>[2x]KFPRVKNWEVGSITYDTLSAQAQQDGPCTPRRCLGSLVFPRKLQGRPSPGPPAPEQLLSQARDFINQYYSSIKRSGSQAHEQRLQEVEAEVAATGTYQLRESELVFGAKQAWRNAPRCVGRIQWGKLQVFDARDCRSAQEMFTYICNHIKYATNRGNLRSAITVFPQRCPGRGDFRIWNSQLVRYAGYRQQDGSVRGDPANVEITELCIQHGWTPGNGRFDVLPLLLQ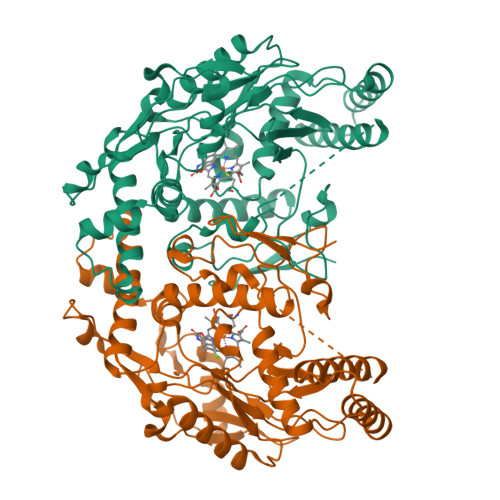APDEPPELFLLPPELVLEVPLEHPTLEWFAALGLRWYALPAVSNMLLEIGGLEFPAAPFSGWYMSTEIGTRNLCDPHRYNILEDVAVCMDLDTRTTSSLWKDKAAVEINVAVLHSYQLAKVTIVDHHAATASFMKHLENEQKARGGCPADWAWIVPPISGSLTPVFHQEMVNYFLSPAFRYQPDPWK>[4x]AFTCHCRRSCYSTEYSYGT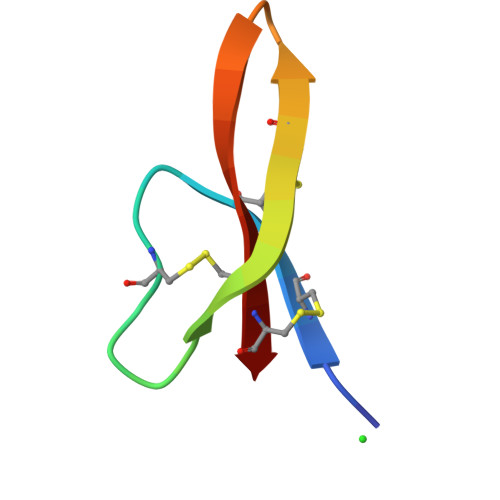CTVMGINWRFCCL>[2x]MSPKVTKEHKDKRQAEILEAAKTVFKRKGFELTTMKDVVEESGFSRGGVYLYFSSTEEMFRRIIETGLDEGLRKLDKSAEHQSVWASISSYLDELTEGLRDVADTLA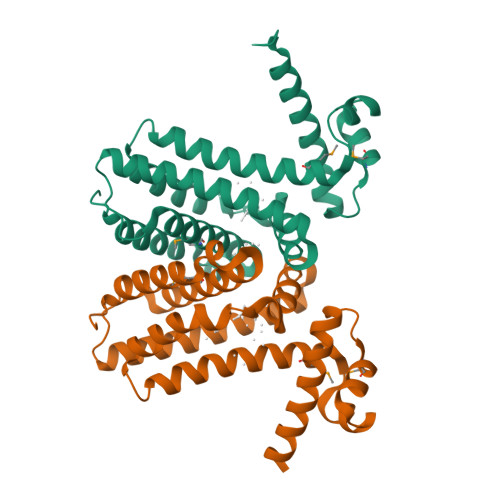PVQFEYLVTAWRNEERRQYLEKRYDLFVERFSRLLQKGIDQGEFQPVQPLATIAKFFLNMNDGIIQNALYFDEEKADVSGLAESAKLYLKTVLQADEK BROMOMETHANE 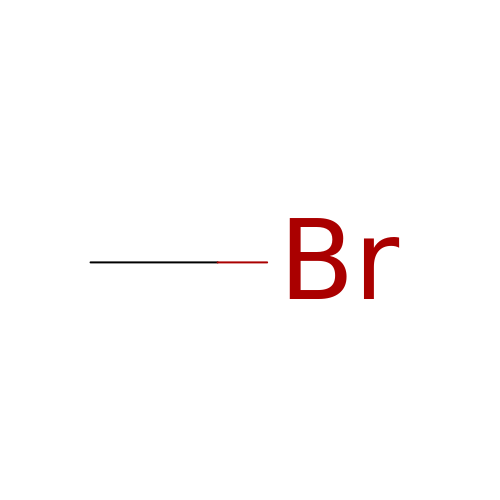| C H3 Br | GZUXJHMPEANEGY-UHFFFAOYSA-N> MQERRALRLGVNGLPNSLEPVNAISNVGPRIVNQIFDTLIARDFFAKGAPGNAIDLVPALAESWERIDEKSVRFKLRQKVMFHDGVELTADDVAYTFSSERLWGPEAIKKIPLGKSYSLDFDEPVVEDKYTVTLRTKTPSYLIETFVASWMSRIVPKEYYKKLGAVDFGNKPVGTGPYKFVEFVAGDRVVLEANDAYWGPKPTASKITYQIVAEPATRVAGLISGEYDIITTLTPDDIQLINSYPDLETRGTLIENFHMFTFNMNQEVFKDKKLRRALALAVNRPIMVEALWKKQASIPAGFNFPNYGETFDPKRKAMEYNVEEAKRLVKESGYDGTPITYHTMGNYYANAMPALMMMIEMWKQIGVNVVMKTYAPGSFPPDNQTWMRNWSNGQWMTDAYATIVPEFGPNGQVQKRWGWKAPAEFNELCQKVTVLPNGKERFDAYNRMRDIFEEEAPAVILYQPYDVYAARKDVHWKPVSFEMMEFRNNLSFGHHHHHH

To our knowledge, the best known system that exemplifies this paradigm is the antibiotic agrocin 84, which penetrates into the cytoplasm of the bacterial pathogen Agrobacterium tumefaciens strain C58 by hijacking the PBP called AccA and its cognate transporter. AccA also plays a key-role in the importation of the characteristic plant tumour-derived compounds such as the opines agrocinopines A and B discovered in 1981 in crown gall tumour tissue. The mature AccA structure is a monomer of 493 residues composed of two lobes, each formed by a central β-sheet flanked by α-helices. We identified the pyranose-2-phosphate-like moiety shared by these two ligands as the key recognition template for AccA.

To address the structural basis for AccA specificity, the carbohydrate fragment of agrocin 84, namely D-glucose-2-phosphate was also synthetized. We determined the structures of AccA in complex with several synthetic derivatives of agrocinopine A and agrocin 84: L-arabinose-2-isopropylphosphate, L-arabinose-2-phosphate and D-glucose-2-phosphate at 2.1, 2.3 and 1.75 Å resolution respectively. L-arabinose relatives and D-glucose-2-phosphate are well defined in the electron density maps. The L-arabinose-2-isopropylphosphate and L-arabinose-2-phosphate alone or within agrocinopine A make the same protein interactions and superimpose well. A similar observation can be made for the bound D-glucose-2-phosphate. To summarize, AccA binds the pyranose-2-phosphate/phosphoramidate key-template through numerous polar interactions and its selectivity for this motif was validated by the structures of AccA in complex with L-arabinopyranose-2-phosphate and D-glucopyranose-2-phosphate. The selectivity of AccA for this ligand motif was validated by the structures of AccA in complex with L-arabinose-2-phosphate and D-glucose-2-phosphate and their affinity measurement. AccA cannot recognize a phosphate alone, nor a D-glucose, nor a L-arabinose, nor a glucose linked to a phosphate via an oxygen atom other than its O2. The D-glucose-2-phosphate moiety of agrocin 84 acts as a ‘molecular passkey’, which is recognized by a large variety of pathogenic agrobacteria expressing the PBP AccA and enzyme AccF.> GMVHYYRLSLKSRQKAPKIVNSKYNSILNIALKNFRLCKKHKTKKPVQILALLQEIIPKSYFGTTTNLKRFYKVVEKILTQSSFECIHLSVLHKCYDYDAIPWLQNVEPNLRPKLLLKHNLFLLDNIVKPIIAFYYKPIKTLNGHEIKFIRKEEYISFESKVFHKLKKMKYLVEVQDEVKPRGVLNIIPKQDNFRAIVSIFPDSARKPFFKLLTSKIYKVLEEKYKTSGSLYTCWS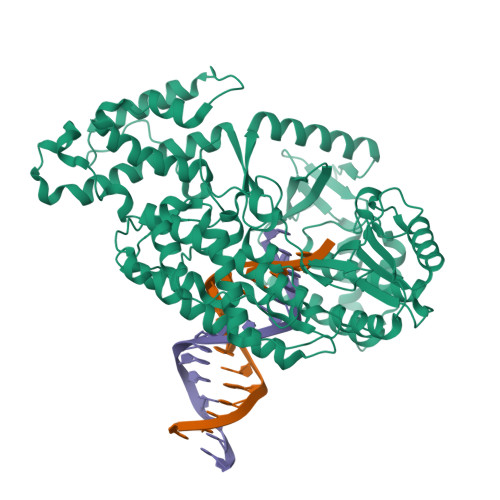EFTQKTQGQIYGIKVDIRDAAGNVKIPVLCKLIQSIPTHLLDSEKKNFIVDHISNQFVAFRRKIYKWNHGLLQGDPLSGCLCELYMAFMDRLYFSNLDKDAFIHRTVDDYFFCSPHPHKVYDFELLIKGVYQVNPTKTRTNLPTHRHPQDEIPYCGKIFNLTTRQVRTLYKLPPNYEIRHKFKLWNFNNQISDDNPARFLQKAMDFPFICNSFTKFEFNTVFNDQRTVFANFYDAMICVAYKFDAAMMALRTSFLVNDFGFIWLVLSSTVRAYASRAFKKIVTYKGGKYRKVTFQCLKSIAWRAFLAVLKRRTEIYKGLIDRIKSREKLTMKFHDGEVDASYFCKLPEKFRFVKINRKASI> MSVLDALWEDRDVRFDLSAQQMKTRPGEVLIDCLD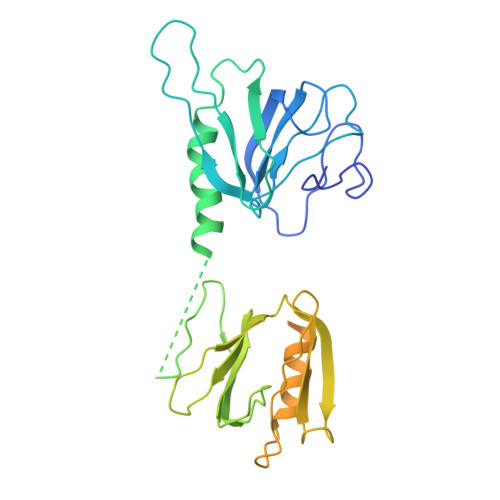SIEDTKGNNGDRGRLLVTNLRILWHSLALSRVNVSVGYNCILNITTRTANSKLRGQTEALYILTKCNSTRFEFIFTNLVPGSPRLFTSVMAVHRAYETSKMYRDFKLRSALIQNKQLRLLPQEHVYDKINGVWNLSSDQGNLGTFFITNVRIVWHANMNDSFNVSIPYLQIRSIKIRDSKFGLALVIESSQQSGGYVLGFKIDPVEKLQESVKEINSLHKVYSASPIFGVDYEMEEKPQPLEALTVEQIQDDVEIDSDGHTDAFVAYFADGNKQQDREPVFSEELGLAIEKLKDGFTLQGLWEVMS>[4x]MHHHHHHLEPPPSTFQPLCHPLVEEVSKEVDGYFLQHWNFPNEKARKKFV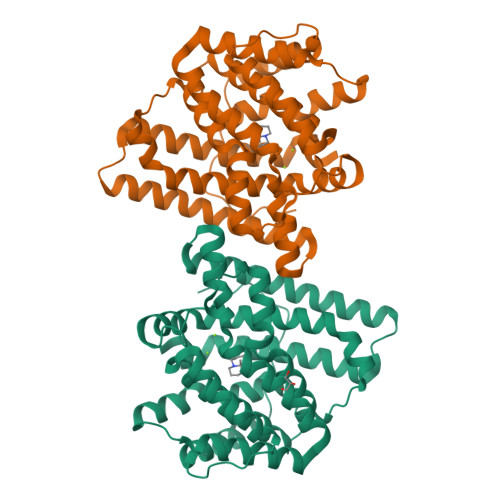AAGFSRVTCLYFPKALDDRIHFACRLLTVLFLIDDLLEYMSFEEGSAYNEKLIPISRGDVLPDRSIPVEYIIYDLWESMRAHDREMADEILEPVFLFMRAQTDRTRARPMGLGGYLEYRERDVGKELLAALMRFSMGLKLSPSELQRVREIDANCSKHLSVVNDIYSYEKELYTSKTAHSEGGILCTSVQILAQEADVTAEAAKRVLFVMCREWELRHQLLVARLSAEGLETPGLAAYVEGLEYQMSGAELWSQTTLRYSVVVD Argonaute-family proteins have crucial roles in gene regulation in collaboration with small guide strands, which recognize complementary sequences in the target. Argonaute proteins belong to the PIWI protein superfamily, and contain a PIWI (P element-induced wimpy testis) domain, a MID (middle) domain, a PAZ (Piwi–Argonaute–Zwille) domain and an N-terminal domain. The Argonaute protein of R. sphaeroides lacks slicer activity and thus permits the formation of Argonaute complexes containing the guide strand and the uncleaved target strand. Our biochemical analysis shows that RsAgo specifically interacts with RNA and DNA as the guide and target strands, respectively, suggesting that RsAgo has a key role in a unique silencing system, that is, RNA-guided DNA silencing.

On the basis of the results of the nucleic acid recognition assay, we crystallized RsAgo complexed with a hybrid duplex containing a 5′P 18-base guide RNA strand and an 18-base complementary DNA target strand, and solved the structure at 2 Å resolution using the single-wavelength anomalous dispersion method with SeMet-labelled proteins. RsAgo was composed of N-terminal, PAZ, MID and PIWI domains, and L1 and L2 linkers. The fully solved heteroduplex is bound within a positively charged channel between N–PAZ-containing and MID–PIWI-containing lobes by an extensive hydrogen-bonding network. Surprisingly, the 3′-region of the guide RNA strand was base-paired with the 5′-region of the target DNA strand; this behaviour has not been reported previously for other Argonaute complexes. In the MID domain, the 5′-phosphate of the guide RNA strand forms hydrogen bonds with the side chains of Y463, K467, Q478, K506 and the main chains of Q479. The aromatic residue Y463 stacked against the 5′-terminal uracil and the main chain of A454 formed a hydrogen bond with N3 of the uracil. The present RNA-guided RsAgo structure showed that a magnesium ion was coordinated by the first and third phosphates of the guide RNA strand and by the carboxyl group of L777. The PAZ domain of RsAgo (R204, R209, G210, L211, E242 and G243) mainly interacted with the middle region (nucleotides 8, 9, 11 and 12) of the guide RNA strand in the heteroduplex. However, the PAZ domain of RsAgo lacks the second subdomain, and therefore does not possess the PAZ pocket. On this surface, the target DNA strand (nucleotides 14′–16′) formed hydrogen bonds with the side chains of K49, R52, H62 and R97, and the main chain of W63.

>MGSSHHHHHHSSGLVPAGSHMQLVSNGFEVNLPDQVEVIVRDLPDPSKVKEERTRLMGYWFVHWFDGKLFHLRIKAGGPNVDGEHRAIRTAEHPWLLRARLDDALEEALPKYAAVKKRPFTFLAQKDELIDAAATAAGLSHRLLNSFKVIPRFALSPKIYEPVDGTTRVGVFVTIGMRYDIEASLRDLLEAGIDLRGMYVVRRKRQPGERGLLGRVRAISDDMVQLFEETDLASVNVNDAKLEGSKENFTRCLSALLGHNYKKLLNALDDQEAGYRTGPRFDDAVRRMGEFLAKKPIRLADNINAQVGDRIVFSNEGQARNVRLAPKVEYVFDRTGAKSAEYAWRGLSQFGPFDRPSFANRSPRILVVYPSSTQGKVENFLSAFRDGMGSNYSGFSKGFVDLMGLTKVEFVMCPVEVSSADRNGAHTKYNSAIEDKLAGAGEVHAGIVVLFEDHARLPDDRNPYIHTKSLLLTLGVPTQQVRMPTVLLEPKSLQYTLQNFSIATYAKLNGTPWTVNHDKAINDELVVGMGLAELSGSRTEKRQRFVGITTVFAGDGSYLLGNVSKECEYEGYSDAIRESMTGILRELKKRNNWRPGDTVRVVFHAHRPLKRVDVASIVFECTREIGSDQNIQMAFVTVSHDHPFVLIDRSERGLEAYKGSTARKGVFAPPRGAISRVGRLTRLLAVNSPQLIKRANTPLPTPLLVSLHPDSTFKDVDYLAEQALKFTSLSWRSTLPAATPVTIFYSERIAELLGRLKSIPNWSSANLNIKLKWSRWFL[2x]> MEHHHHHHMPVFHTRTIESILEPVAQQISHLVIMHEEGEVDGKAIPDLTAPVAAVQAAVSNLVRVGKETVQTTEDQILKRDMPPAFIKVENACTKLVQAAQMLQSDPYSVPARDYLIDGSRGILSGTSDLLLTFDEAEVRKIIRVCKGILEYLTVAEVVETMEDLVTYTKNLGPGMTKMAKMIDERQQELTHQEHRVMLVNSMNTVKELLPVLISAMKIFVTTKNSKNQGIEEALKNRNFTVEKMSAEINEIIRVLQLTSWDEDA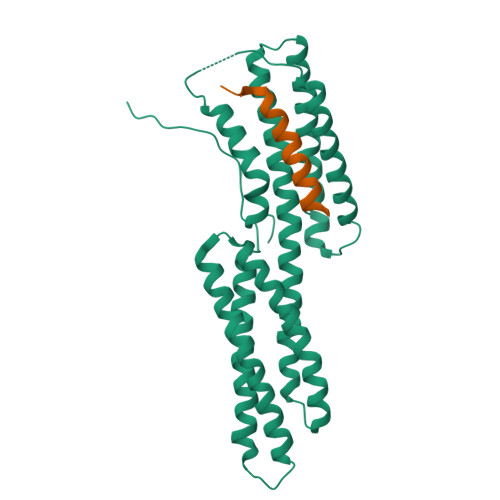W;> AIYEKAKEVSSALSKVLSKIDDT> MRKIVINGGLPLQGEITISGAKNSVVALIPAIILADDVVTLDCVPDISDVASLVEIMELMGATVKRYDDVLEIDPRGVQNIPMPYGKINSLRASYYFYGSLLGRFGEATVGLPGGCDLGPRPIDLHLKAFEAMGATASYEGDNMKLSAKDTGLHGASIYMDTVSVGATINTMIAAVKANGRTIIENAAREPEIIDVATLLNNMGAHIRGAGTNIIIIDGVERLHGTRHQVIPDRIEAGTYISLAAAVGKGIRINNVLYEHLEGFIAKLEEMGVRMTVSE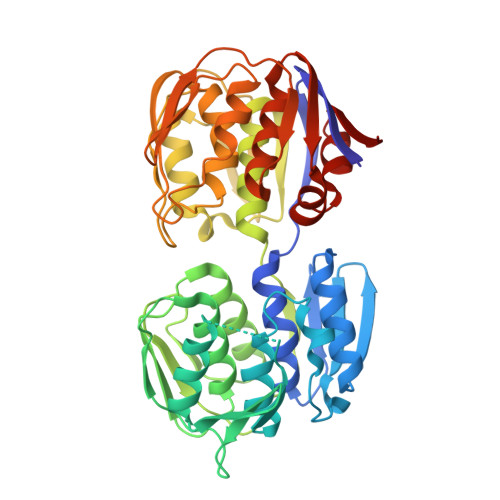DSIFVEEQSNLKAINIKTAPYPGFATDLQQPLTPLLLRANGRGTIVDTIYEKRVNHVFELAKMDADISTTNGHILYTGGRDLRGASVKATDLRAGAALVIAGLMAEGKTEITNIEFILRGYSDIIEKLRNLGADIRLVED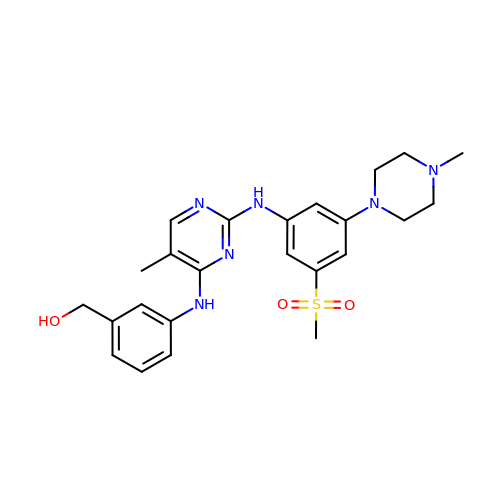[3-[[5-methyl-2-[[3-(4-methylpiperazin-1-yl)-5-methylsulfonyl-phenyl]amino]pyrimidin-4-yl]amino]phenyl]methanol | C24 H30 N6 O3 S | WKJVLTJTBZVAKC-UHFFFAOYSA-N>[12x]MKYVVVSGGVISGIGKGVLASSTGMLLKTLGLKVTSIKIDPYMNIDAGTMSPLEHGECFVLDDGGETDLDLGNYERYLGITLSRDHNITTGKIYSHVISRERRGDYLGKTVQIVPHLTNAIQDWIQRVSKIPVDDTGLEPDVCIIELGGTVGDIESAPFVEALRQFQFEVGRENFALIHVSLVPVIHGEQKTKPTQAAIKDLRSLGLIPDMIACRCSEELNRSTIDKIAMFCHVGPEQVVNVHDVNSTYHVPLLLLKQHMIDYLHSRLKLGEVPLTLEDKERGSQLLTNWENMTKNLDDSDDVVKIALVGKYTNLKDSYLSVTKSLEHASMKCRRQLEILWVEASNLEPETQEVDKNKFHDSWNKLSSADGILVPGGFGTRGIEGM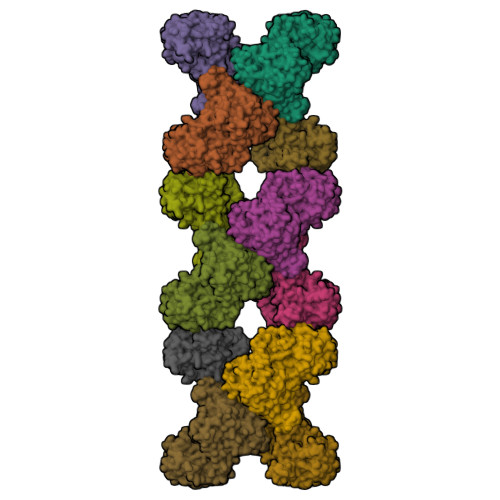ILAAKWARESGVPFLGVCLGLQVAAIEFARNVIGRPNSSSTEFLDETLLAPEDQVVITMRLGLRPTIFQPNSEWSNIRKLYGEVNEVHERHRHRYEINPKIVNDMESRGFIFVGKDETGQRCEIFELKGHPYYVGTQYHPEYTSKVLEPSRPFWGLVAAASGTLGEVIKDINL>MRRYRPTNLEPGDAGIYHHEGHRIRLTKDGRCIITCKTVEVYADESMTVDTPRTTFTGDVEIQKGLGVKGKSQFDSNITAPDAIINGKSTDKHIHRGD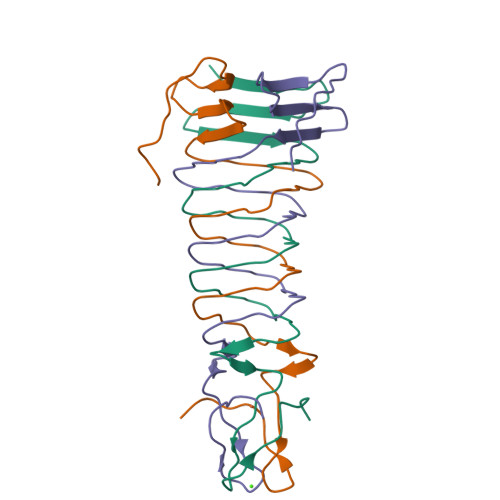SGGTTGPMQLEHHHHHH[6x]> GGCGGAACCGGUGAGUACACCGGAAUCCGAAA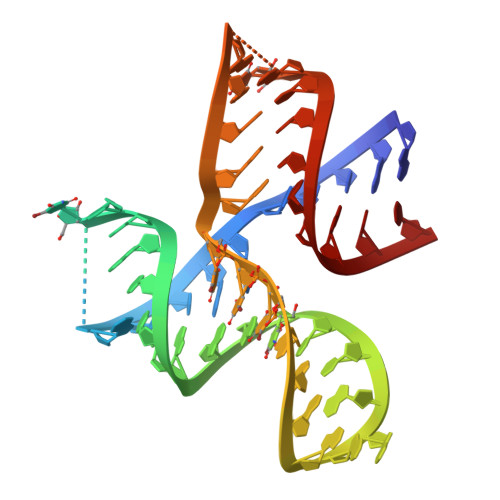GGAUUUGGGCGUGCCCCCGCC>[2x]GPLGSVEEIRLPRAGGPLGLSIVGGSDHSSHPFGV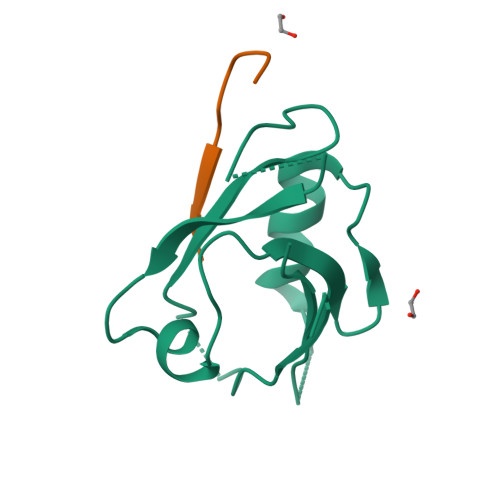QEPGVFISKVLPRGLAARSGLRVGDRILAVNGQDVRDATHQEAVSALLRPCLELSLLVRRD;>TSRQATESTV[2x]[4-(propan-2-yl)piperazin-1-yl](thiophen-2-yl)methanone 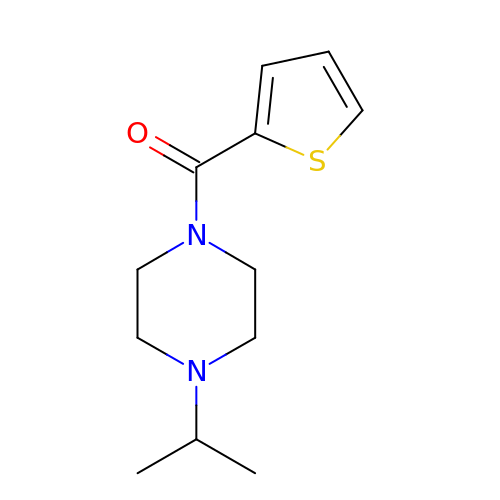| C12 H18 N2 O S | ZEVVAPJSMUTCRY-UHFFFAOYSA-N>[4x]MSKWTYFGPDGENSWSKKYPSCGGLLQSPIDLHSDILQYDASLTPLEFQGYNLSANKQFLLTNNGHSVKLNLPSDMHIQGLQSRYSATQLHLHWGNPNDPHGSEHTVSGQHFAAELHIVHYNSDLYPDASTASNKSEGLAVLAVLIEMGSFNPSYDKIFSHLQHVKYKGQEAFVPGFNIEELLPERTAEYYRYRGSLTTPPCNPTVLWTVFRNPVQISQEQLLALETALYCTHMDDPSPREMINNFRQVQKFDERLVYTSFSQ

The carbonic anhydrase (CA) family (CA, EC 4.2.1.1), consisting of twelve catalytically active human isozymes, performs the catalysis of reversible hydration of CO2 into bicarbonate and acid protons. Since it has been observed that CAIX isozyme is highly overexpressed in numerous cancers, it has been postulated that compounds inhibiting CAIX may possess the anticancer activity and may be used in tumor treatment. Here we have designed a series of compounds, methyl 5-sulfamoyl-benzoates, which bear a primary sulfonamide group, a well-known marker of CA inhibitors, and determined their affinities for all twelve CA isozymes. Eight crystal structures of CA complexes with compounds are presented in this study: 9a bound to CAI and CAII, 3b, 3d, 5b, and 9a bound to CAXII, 3b bound to CAIX and mimic-CAIX (mutant of CAII containing amino acids in the active site as in CAIX: A65S, N67Q, I91L, F130V, V134L, and L203A).

We divided the compounds bound to CAXII into pairs according to their similar binding affinity. Compounds 5b and EA3-3 in the active site of CAXII were compared in Figure 3C. The 5b is well defined in the crystal structure. The binding affinities of the two compounds for CAXII differed by a factor of 2.5, which is insignificant: Kd_intr = 0.020 nM, ΔGintr = −63.5 kJ/mol (5b) and Kd_intr = 0.0080 nM, ΔGintr = −66.0 kJ/mol (EA3-3). These compounds differ structurally by meta-substituents; EA3-3 has a longer and more flexible substituent (-NH(CH2)2OH), but both meta- groups were mostly exposed to the solvent, so they did not contribute much to the positioning in the active site. In addition, the para-cyclooctyl groups of both compounds occupied the same position. Since the chlorinated compounds had less freedom in the active site, the differences in entropy and enthalpy of the slightly different binding of the meta- groups compensated each other: ΔHintr = −43.6 kJ/mol, -TΔSintr = −19.9 kJ/mol (5b) ΔHintr = −39.5 kJ/mol, -TΔSintr = −26.5 kJ/mol (EA3-3). The transition from 1 to 3b and 5b shows different changes in affinity and selectivity; compound 3b bound distinctly more strongly to CAIX (−17.5 kJ/mol), CAXII (-11.4 kJ/mol), whereas compound 5b bound more strongly to CAI (−12.6 kJ/mol), CAVB (−13.3 kJ/mol) and CAXII (−12.6 kJ/mol). Therefore, regardless of the compound, all ortho-compounds occupied a similar position in CAIX and CAXII, and para- occupied another but similar position to each other in CAII and CAXII (respectively).>[2x]MSNAALATAPHALELDVHPVAGRIGAEIRGVKLSPDLDAATVEAIQAALVRHKVIFFRGQTHLDDQSQEGFAKLLGEPVAHPTVPVVDGTRYLLQLDGAQGQRANSWHTDVTFVEAYPKASILRSVVAPASGGDTVWANTAAAYQELPEPLRELADKLWAVHSNEYDYASLKPDIDPAKLERHRKVFTSTVYETEHPVVRVHPISGER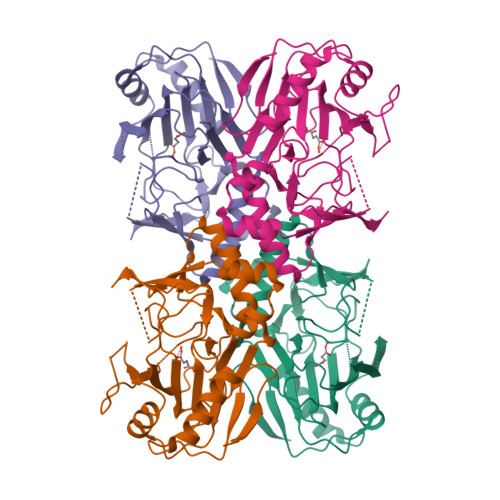ALQLGHFVKRIKGYSLADSQHLFAVLQGHVTRLENTVRWRWEAGDVAIWDNRATQHYAVDDYGTQPRIVRRVTLAGEVPVGVDGQLSRTTRKG Class A plexins (PlxnAs) act as semaphorin receptors and control diverse aspects of nervous system development and plasticity, ranging from axon guidance and neuron migration to synaptic organization. Plexins are large type 1 transmembrane proteins comprising typically ten domains in their extracellular segment, a single membrane spanning region that is predicted to be helical and a conserved, cytoplasmic region that contains a GTPase-activating protein (GAP) domain with a Rho GTPase-binding domain insert. All our PlxnA ectodomain structures show autoinhibitory, intermolecular “head-to-stalk” (domain 1 to domain 4-5) interactions, which are confirmed by biophysical assays, live cell fluorescence microscopy, and cell-based and neuronal growth cone collapse assays. This work reveals a 2-fold role of the PlxnA ectodomains: imposing a pre-signaling autoinhibitory separation for the cytoplasmic domains via intermolecular head-to-stalk interactions and supporting dimerization-based PlxnA activation upon ligand binding.

The membrane proximal domain IPT6 (domain 10) is positioned perpendicular to the ring formed by domains 1 to 9, and the IPT6 C terminus points away from the plane of the ring. This out-of-the-ring orientation of IPT6 is observed in all five PlxnA ectodomain structures for which the electron density is sufficiently well ordered to allow IPT6 to be resolved. The same relative domain orientation recurs in the structure of PlxnA17-10. Possibly this distinctive orientation is stabilized by a loop (1,175–1,184) extending from IPT6 that provides hydrophobic interactions with three residues in domain IPT5, Trp1055, Ile1057, and Tyr1145, which are conserved across the A class Plxns. In the full-length plexin, the linker between IPT6 and the transmembrane helix is predicted to be short (6 residues for PlxnA1), and thus, for this conformation, the plexin extracellular segment is most likely positioned close to the membrane with its ring parallel to the cell surface. The interface between PSI3 and IPT3 (domains 6 and 7) differs markedly from those of PSI1-IPT1 and PSI2-IPT2, imposing a more acute angle on the relative arrangement of these two domains, and thus reducing the ring circumference.

> ETGDPKILKLSPETGPRQGGTRLTITGENLGLRFEDVRLGVHVGKVLCSPVESEYISAEQIVCEIGDASTLRAHDALVEVCVRDCSLHYRALSPKRFTFVTPTFYRVSPSRGPLSGGTWIGIEGSHLNAGSDVAVSIGGRPCSFSWRNSREIRCLTPPGHTPGSAPIVININRAQLSNPEVKYNYTEDPTILRIDPEWSINSGGTLLTVTGTNLATVREPRIRAKYGGIERENSCMVYNDTTMVCRAPSIDNPKRSPPELGERPDEIGFIMDNVRTLLVLNSSSFLYYPDPVLEPLSPTGLLELKPSSPLILKGRNLLPPAPGNSRLNYTVLIGSTPCILTVSETQLLCEAPNLTGQHKVTVRAGGFEFSPGMLQVYSDSLLTLGTKHHHHHH>MGSSHHHHHHSSGLVPAGSHSKVFIRSAINRVHQNSAANGGELPRIVFPEGTSTKVLKALATLVEEKICQPILLGYPERVKEKIKALDIPLLNDVSIVHPSSHPKYFSFVEKLYSLRQRKGINLGRAERLMADPNYFAAMMVNQGEADGMVSGSSINYADAVRPILQTIGVYKEGIPAGLNFVLLEDKFLVLADTTVNLNPTAEQCAQIALQAAKIVEYFGIEPRVAMLSYSNFSGAEGTPRKMKKAAEIARSLRPDLM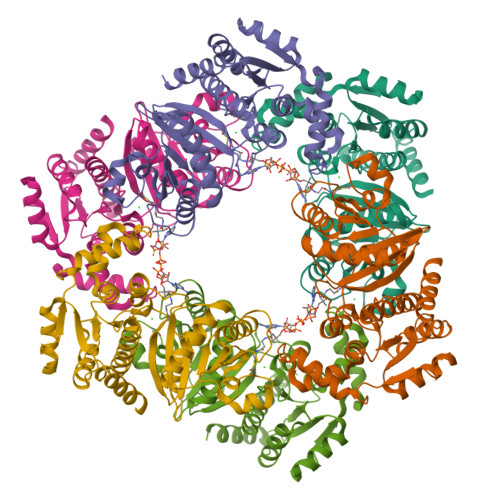IEGDMQADTAVNPEIMERLFPFSGLKGGANVLVFPNLESSNIAYKLIQQIGKAEVIGPFLTGVRRSANVLQRTTTVDGIVNSVVFTALEAQYIKEVLKSRGKK[6x]> MKYIIANWKAHKTLEEASAWVDSVNKQISQTPDVQRKLEDDELIILIAAPFPFLVPLSQKISQKNLAVAAQDVSVYGEGAYTGEVTAKMLKGVTTHVLIGHSERKDYFHETDEVVLKKSEQVLSQGLSPIFCIQNESNKIPEGANII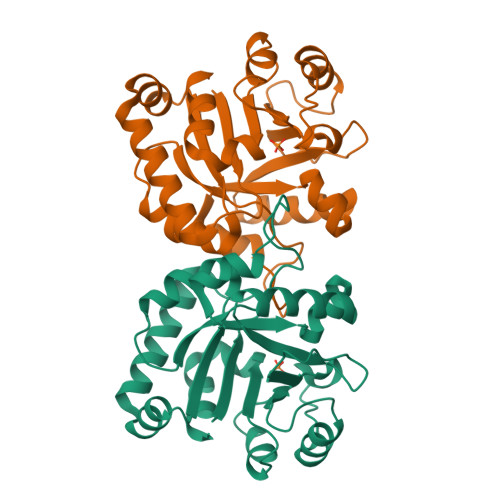AYDPKEAIGTGKNVPGEETATFRKKLNLFPDAVFLYGGSVNPESIDEYLSHPEINGFLVGGSSLDPEEFFELVKKL>MKKRVVKLRELVPAVAALAVAVLIQSATGSSGGSGHTPTTQATHADDHDLTTHNGTEEHDDGHDDGHDDLHAHAPKVIVFISGSCLFGAISRSLFKKLPIPYTVVLLILGAILGVVASNVPLVEEHTRDVAHMDPHVLLQIFLPVLIFESAFAMDVHTFMRSFSQVCILALFGLVVASVLTAVLAMNLFNYNWNFSEAMMFGAIMSATDPVAVVALLKDLGASKQLGTIIEGESLLNDGCAIVIFNVFMKMVFFPQLTSTVGQNVLYFLQVAVAGPLWGYAVAKVTVFFLSHIFNDALVEITITLAATYLTYYIGDIWLEVSGVLAVVVLGLIVNAEKTSISPEVEVFLHRFWEMLAYLANTLIFMMVGVVVTQKALVAVDKMDWFYLIILYLAITIIRGMVISLFSPILSRIGYGLTWRNAVIMTWGGLRGAVGLALALVVENLAGNDVIGSKFLFHTAGIVVLTLVINATTIQTLLRILGMSDISIPKRLAMAGAVRRIHEGQNRTLNMLKSDRFLADADWDIATAACEISDPYSALSDDENAPADELTLGERKSVCPGCKAMVPNEPSPREFADMMEEARLRMLKAEKISYWKQFEHGMLAREALRLLVQHAEVAADEKDQFILVDDLKKSWQIKGIYPWLKRKLEDLISEKKIAAIPMPKYKLGKLMYKICHHMAFEVTINIAIVLNIVPIIMEFVVQDKMASVSTMAAPGSTVSSEPSSLQKIEDALRISNYVFFVIYAIEAIVKILGLGRHYIVSHWNKFDAFILVVALVDIIIAETLLKGSITINLSSIKVVKLFRLLRGLRMLRLTKALIPKLILVVNGKINNQLSLGYDVGKGYIIGEEEVGKIIDRMVDNKKILRELKHISETGRLQVVKELGLLQREHPGIAVSVKTRQAIRTILNHSRETIHELQGAGLLDEMEAHKLELTVEIKMKRLMNAPSSIPPPPPENLLKNVSWLAGDMKLIDFIKARASLLHFDYGEVIVREGDESDGLFLIVSGLVKLYGKSAFLDHDNPPVTAGSEENEVFEDYLTVGNVIGEMGVLTKKPRNATVTCETTVQVYFITAEDMNIAIDTFTLYPSLEYRLWRVVAIRIATPLIMEQMAFQGWTQEKVKLHLERGYLVDLAESHFQFNIDATLEDVILINGTAYNAHTREEIRSPCLISRTVHKLTFQYTATEEPRLFVVRNAEYNGPILDGRLDVDSKRSLISITEISSNMCLKHAAELRQKNSKVMLSRKSSGAAAKEEEDCIPNTSDVEQAAGVSPSVPTKTTPKPKSFLPSLGLSMSKERVNGEAVEESPVKTKQGEETPETEEGAAPRVNVENLYFQ[2x]

SLC9C1 belongs to the NHE family of ion transporters, which facilitate the electroneutral exchange of cations (Na+/Li+/K+) and protons (H+) across membranes to regulate intracellular pH, sodium levels and cell volume. Rather than containing a partially disordered cytoplasmic tail, it contains four additional TM helices that form an S1–S4 voltage-sensing domain (VSD), and a distal cyclic-nucleotide-binding domain (CNBD)2,4. The S4 VSD renders SLC9C1 a transporter that is activated only in response to hyperpolarization (−95 mV), and the CNBD bind cAMP to enable SLC9C1 to become activated closer to the resting membrane potential of sperm (−50 mV)2 VSDs are thought to have evolved independently from ion channels, and there are a few examples of non-channel VSD domains coupled to soluble enzymes. SLC9C1 is therefore an essential component of the pH–sAC–cAMP signalling pathway in metazoa, required for sperm motility and fertilization.

The maps obtained in nanodiscs showed poor map density for the VSDs. With a subset of particles processed in C1 symmetry, the map density of the VSD in nanodiscs was improved to confirm the same overall positioning of the VSD as in detergent, but with no clear side-chain map density. The cryo-EM maps for the transporter module were at a higher resolution in some regions of the nanodisc reconstruction, with a local resolution of up to 2.5 Å in most regions. In the nanodisc structure, cryo-EM map density at a local resolution of 2.5 Å supported the modelling of two phosphatidic acid (PA) lipids at the dimerization interface. The presence of PA lipids probably stabilized a more compacted SLC9C1 homodimer in the nanodisc structure, which was evident by the repositioning of helices at the dimerization interface. However, in the presence of PA, His73 interacts with the lipid, and the TM2′–TM3′ extracellular region has rearranged to coordinate the PA headgroup through water-bridged His132 and Asp129. The lipid-induced rearrangement observed in SLC9C1 is centred around an extracellular helical motif (ECH1) that is not present in the NHE119, NHE335 and NHE918 structures. In DDM/CHS, the SLC9C1 protein migrated as both a dimer and monomer. The purified SLC9C1 protein was further heated at 45 °C for 10 min in the presence of PA, PC, PS or PE lipid, yet only the addition of PA improved the resistance of SLC9C1 to heat denaturation.>[6x]AMNNTIINSLIGGDDSIKRSNVFAVDSQIPTLYMPQYISLSGVMTNDGPDNQAIASFEIRDQYITALNHLVLSLELPEVKGMGRFGYVPYVGYKCINHVSISSCNGVIWEIEGEELYNNCINNTIALKHSGYSSELNDISIGLTPNDTIKEPSTVYVYIKTPFDVEDTFSSLKLSDSKITVTVTFNPVSDIVIRDSSFDFETFNKEFVYVPELSFIGYMVKNVQIKPSFIEKPRRVIGQINQPTATVTEVHAATSLSVYTKPYYGNTDNKFISYPGYSQDEKDYIDAYVSRLLDDLVIVSDGPPTGYPESAEIVEVPEDGIVSIQDADVYVKIDNVPDNMSVYLHTNLLMFGTRKNSFIYNISKKFSAITGTYSDATKRTIFAHISHSINIIDTSIPVSLWTSQRNVYNGDNRSAESKAKDLFINDPFIKGIDFKNKTDIISRLEVRFGNDVLYSENGPISRIYNELLTKSNNGTRTLTFNFTPKIFFRPTTITANVSRGKDKLSVRVVYSTMDVNHPIYYVQKQLVVVCNDLYKVSYDQGVSITKIMG

In Vaccinia virus (VACV), copies of the double-jelly-roll protein D13 bind to the viral membrane via interaction with its partner protein A17 and assemble into a scaffold surrounding the viral membrane. This process leads to the formation of a spherical immature virion (IV). The 62-kDa D13 protein exists as trimers both in vivo and in vitro, and structures of the recombinantly expressed D13 trimer have been determined by X-ray crystallography. D13 adopts a double-jelly-roll structure composed of 8 antiparallel β-strands.

Image processing of D13 trimers revealed a small subpopulation of adjacent trimers bound together, forming doublets of trimers. Although the resolution of the resulting 3D reconstruction (3.9 Å on average) was not fully isotropic, it allowed unambiguous positioning of an atomic model for identification of the intertrimer interfaces. There are two major interfaces that mediate doublet formation. The first is located between one of the head domains on each of the two trimers. Side chains of R353 in the EFH loop and D325 in the CDH loop extend toward each other, suggesting salt bridge interactions. Another interface is located at the base of the trimers, which would be proximal to the viral membrane in the IV. At this interface, the major difference of doublet structure in comparison to the singlet trimer is the unambiguous absence of the N-terminal tail α-helix. The clearly resolved features in the reconstructed electron potential map between Y62 and R498 suggests cation-π interactions as the main stabilizer at this interface. Furthermore, the doublet is characterized by a slight twist of the trimer axes defined by a torsion angle of 8.0°, leading to an arched arrangement when the doublets are linearly expanded. The absence of the N-terminal tail α-helix in the doublet structure suggests that its displacement likely helps to initiate intertrimer interactions, promoting ordered assembly of oligomers and leading to formation of spherical IV-like particles.>[4x]MEAEQRPAAGASEGATPGLEAVPPVAPPPATAASGPIPKSGPEPKRRHLGTLLQPTVNKFSLRVFGSHKAVEIEQERVKSAGAWIIHPYSDFRFYWDLIMLLLMVGNLIVLPVGITFFKEENSPPWIVFNVLSDTFFLLDLVLNFRTGIVVEEGAEILLAPRAIRTRYLRTWFLVDLISSIPVDYIFLVVELEPRLDAEVYKTARALRIVRFTKILSLLRLLRLSRLIRYIHQWEEIFHMTYDLASAVVRIFNLIGMMLLLCHWDGCLQFLVPMLQDFPPDCWVSINHMVNHSWGRQYSHALFKAMSHMLCIGYGQQAPVGMPDVWLTMLSMIVGATCYAMFIGHATALIQSLDSSRRQYQEKYKQVEQYMSFHKLPADTRQRIHEYYEHRYQGKMFDEESILGELSEPLREEIINFTCRGLVAHMPLFAHADPSFVTAVLTKLRFEVFQPGDLVVREGSVGRKMYFIQHGLLSVLARGARDTRLTDGSYFGEICLLTRGRRT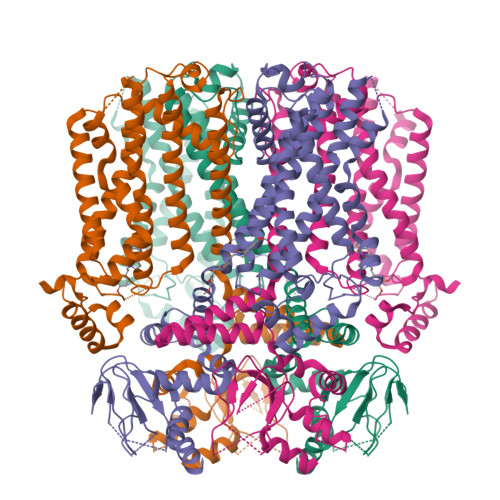ASVRADTYCRLYSLSVDHFNAVLEEFPMMRRAFETVAMDRLLRIGKKNSILQRKRSEPSPGSSGGIMEQHLVQHDRDMARGVRGRAPSTGAQLSGKPVLWEPLVHAPLQAAAVTSNVAIALTHQRGPLPLSPDSPATLLARSAWRSAGSPASPLVPVRAGPWASTSRLPAPPARTLHASLSRAGRSQVSLLGPPPGGGGRRLGPRGRPLSASQPSLPQRATGDGSPGRKGSGSERLPPSGLLAKPPRTAQPPRPPVPEPATPRGLQLSANM> MSKATEQNDKLKRAIIISAVLHVILFAALIWSSFDENIEASAGGGGGSSIDAVMVDSGAVVEQYKRMQSQESSAKRSDEQRKMKEQQAAEELREKQAAEQERLKQLEKERLAAQEQKKQAEEAAKQAELKQKQAEEAAAKAAADAKAKAEADAKAAEEAAKKAAADAKKKAEAEAAKAAAEAQKKAEAAAAALKKKAEAAEAAAAEARKKAATEAAEKAKAEAEKKAAAEKAAADKKAAAEKAAADKKAAEKAAAEKAAADKKAAAEKAAADKKAAAAKAAAEKAAAAKAAAEADDIFGELSSGKNAPKTGGGAKG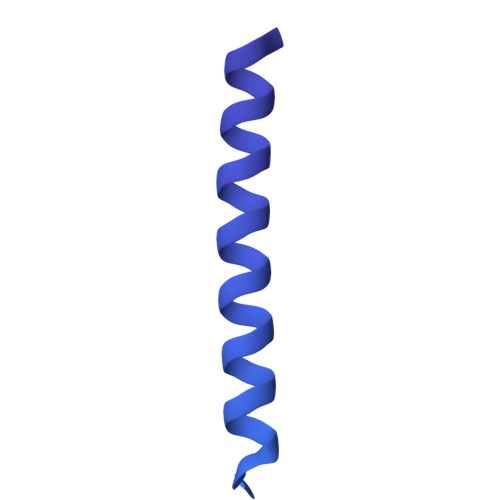NNASPAGSGNTKNNGASGADINNYAGQIKSAIESKFYDASSYAGKTCTLRIKLAPDGMLLDIKPEGGDPALCQAALAAAKLAKIPKPPSQAVYEVFKNAPLDFKP>[4x]GSMSTINFANREINFKIVYYGPGLSGKTTNLKWIYSKVPEGRKGEMVSLATEDERTLFFDFLPLDIGEVKGFKTRFHLYTVPGQVFY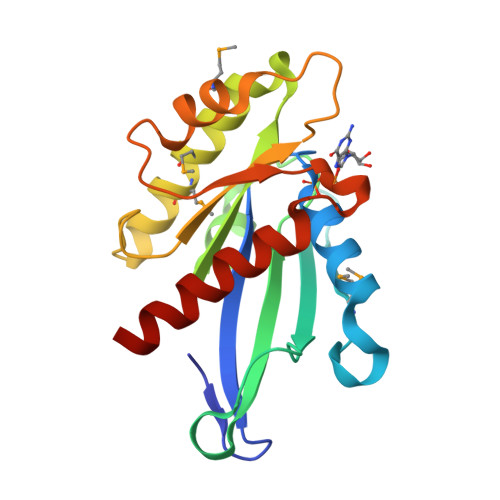NASRKLILRGVDGIVFVADSAPNRLRANAESMRNMRENLAEYGLTLDDVPIVIQVNKRDLPDALPVEMVRAVVDPEGKFPVLEAVATEGKGVFETLKEVSRLVLARVAGGS> MHHHHHHHDGTENPIHDRTSDYHKYLKVKQGDSDLFKLTVSDKRYIWYNPDPKERDSYECGEIVSETSDSFTFKTVDGQDRQVKKDDANQRNPIKFDGVEDMSELSYLNEPAVFHNLRVRYNQDLIYTYSGLFLVAVNPFKRIPIYTQEMVDIFKGRRRNEVAPHIFAISDVAYRSMLDDRQNQSLLITGESGAGKTENTKKVIQYLASVAGRNQANGSGVLEQQILQANPILEAFGNAKTTRNNNSSRFGKFIEIQFNSAGFISGASIQSYLLEKSRVVFQSETERNYHIFYQLLAGATAEEKKALHLAGPESFNYLNQSGCVDIKGVSDSEEFKITRQAMDIVGFSQEEQMSIFKIIAGILHLGNIKFEKGAGEGAVLKDKTALNAASTVFGVNPSVLEKALMEPRILAGRDLVAQHLNVEKSSSSRDALVKALYGRLFLWLVKKINNVLCQERKAYFIGVLDISGFEIFKVNSFEQLCINYTNEKLQQFFNHHMFKLEQEEY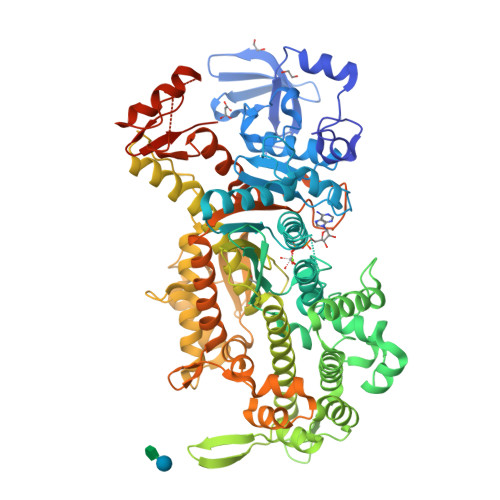LKEKINWTFIDFGLDSQATIDLIDGRQPPGILALLDEQSVFPNATDNTLITKLHSHFSKKNAKYEEPRFSKTEFGVTHYAGQVMYEIQDWLEKNKDPLQQDLELCFKDSSDNVVTKLFNDPNIASRAKKGANFITVAAQYKEQLASLMATLEAANPHFVRCIIPNNKQLPAKLEDKVVLDQLRCNGVLEGIRITRKGFPNRIIYADFVKRYYLLAPNVPRDAEDSQKATDAVLKHLNIDPEQYRFGITKIFFRAGQLARIEEAREQRLESNEPPMDFDDDIPF> MKKIYFMLAIAGIFAGCVPSANSATKNSSANSTAPSQDVIVQKVDKDDVRDIIREEKMLAPDASETELSFTAVGEGI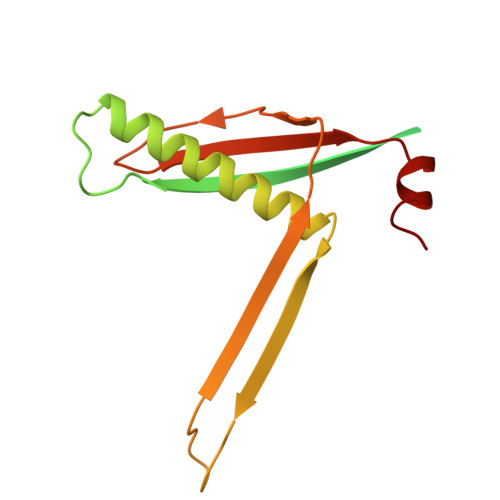APMNTVSTAQALALAKRAAITDAYRQLASKLYGVKVNGKDTVKDAMLRSSTITAQVNGLIKNASIIDENFNQGLYRVNLELKIDADKWKELFAY> RNSPEDK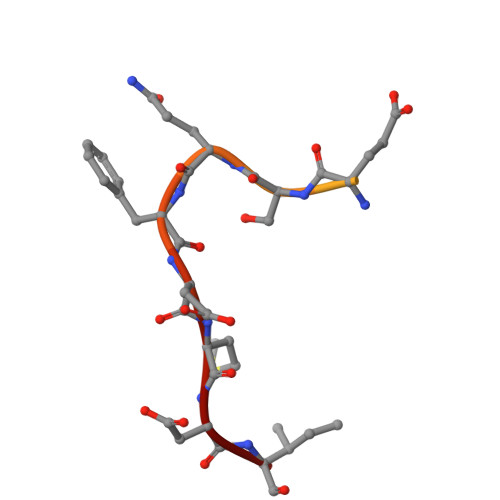RAGGEESQFEMDI>[7x]VEKNITVRASVDPKLDLLQADGTSLPDSIALTYSSASNNFEVYSLNTAIHTNDKSKGVVVKLSASPVLSNIMKPNSQIPMKVTLGGKTLNTTDTE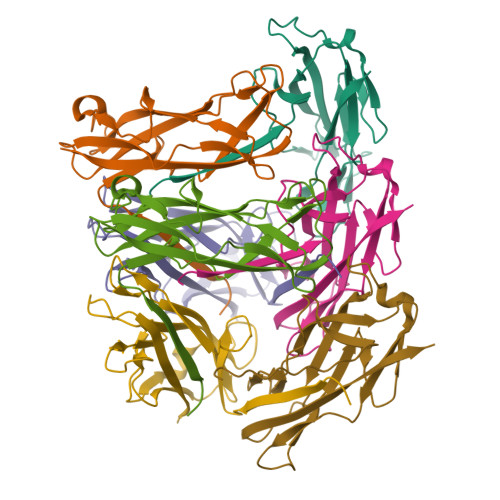FTVDTLNFGTSGVENVSSTQQLTIHADTQGTAPEAGNYQGIISLIMTQKT> IVGGYECTKHSQAHQVSLNSGYHFCGGSLVSKDWVVSAAHCYKSVLRVRLGEHHIRVNEGTEQYISSSSVIRHPNYSSYNINNDIMLIKLTKPATLNQYVHAVALPTECAADATMCTVSGWGNTMSSVADGDKLQCLSLPILSHADCANSYPGMITQSMFCAGYLEGGKDSCQGDSGGPVVCNGVLQGVV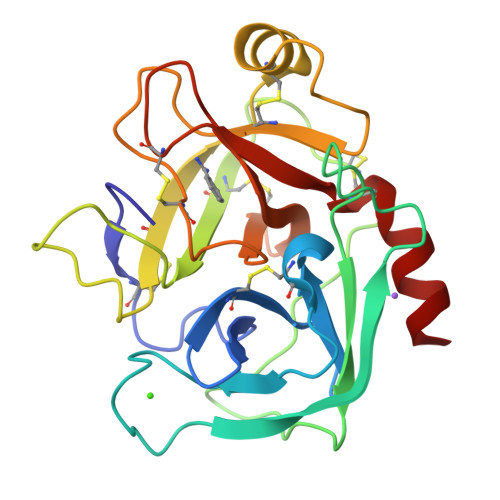SWGYGCAERDHPGVYAKVCVLSGWVRDTMA> PELELKYLNMMKMAITG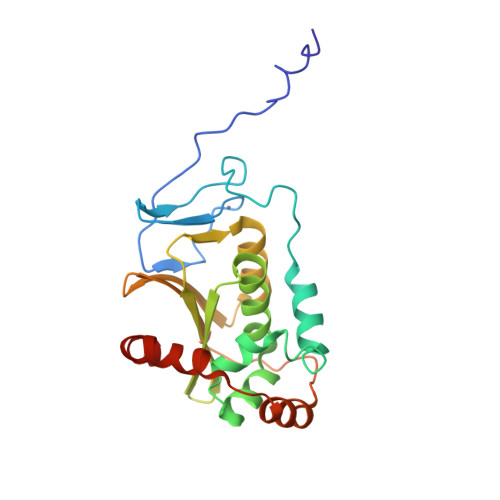KESICLPFNFHSHRQHTCLDISPYGNEQVSRIACTSCEDNRILPTASDAMVAFINQTSNIMKNRNFYYGFCKSSELLKLSTNQPPIFQIYYLLHAANHDIVPFMHAEDGRLHMHVIFENPDVHIPCDCITQMLTAAREDYSVTLNIVRDHVVISVLCHAVSASSVKIDVTILQRKIDEMDIPNDVSESFERYKELIQELCQS> SHMAPTITFLESPTSDHHWCIPFTVKGNPKPALQWFYNGAILNESKYICTKIH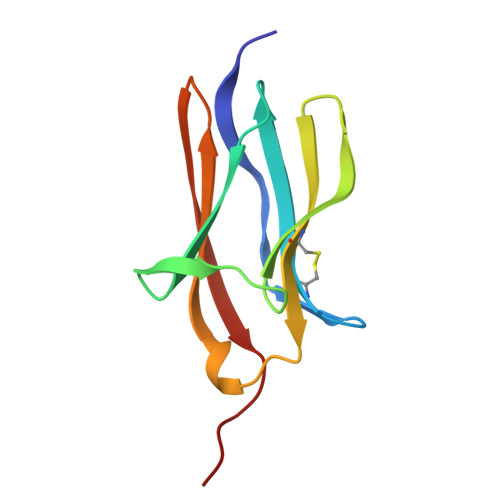VTNHTEYHGCLQLDNPTHMNNGDYTLIAKNEYGKDEKQISAHFMGWPG>KETAAAKFERQHMDSSTSAASSSNYCNQMMKSRNLTKDRCKPVNTFVHESLADVQAVCSQKNVACKNGQTNCYQSYS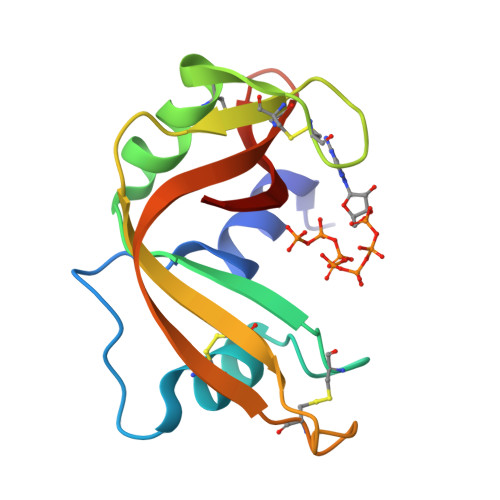TMSITDCRETGSSKYPNCAYKTTQANKHIIVACEGNPYVPVHFDASV[2x]2-amino-4-oxo-N-(1H-1,2,3-triazol-5-ylmethyl)-1,4-dihydropteridine-7-carboxamide | C10 H9 N9 O2 | 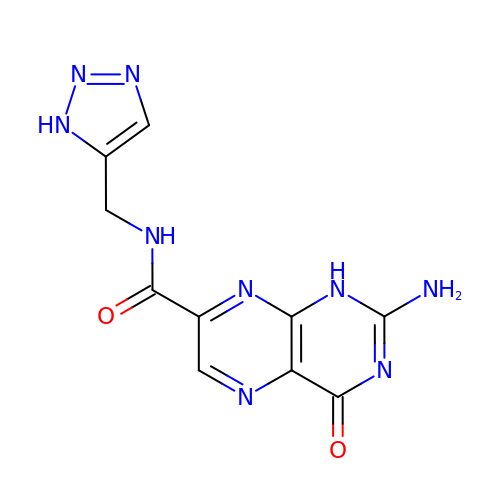IOLZYHQWMHJFBL-UHFFFAOYSA-N> MRGSHHHHH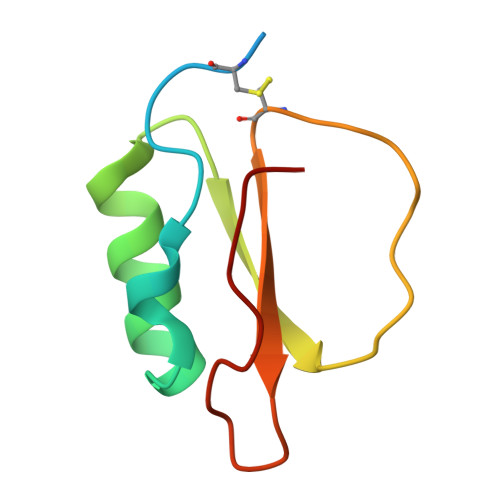HLRQCSGKQEWPELVGERGSKAAKIIENENEDVRAIVLPEGSAVPRDLRCDRVWVFVDERGVVVDTPVVM> FADDHAMSPDMKLLAGASNWVNQSGSVAQFVFTPSPTQPQTYEVSGNYINNAQGTGCKGTPYPLSGAYYSGNQIISFSVVWSNASANCQSATGWTGYFDFSGSQAVLKTDWNLAFYSGSTPAIQQ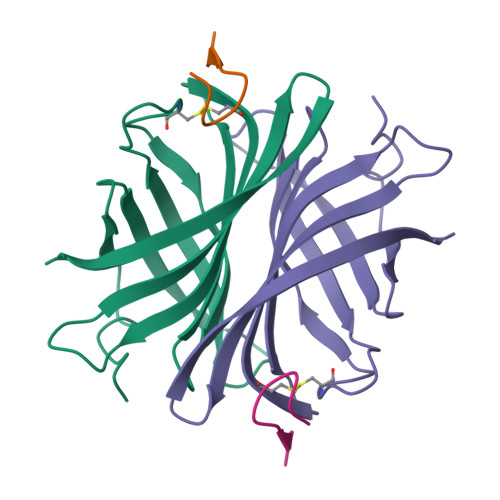GQDDFMQSV;> SVATVSESLLTE> E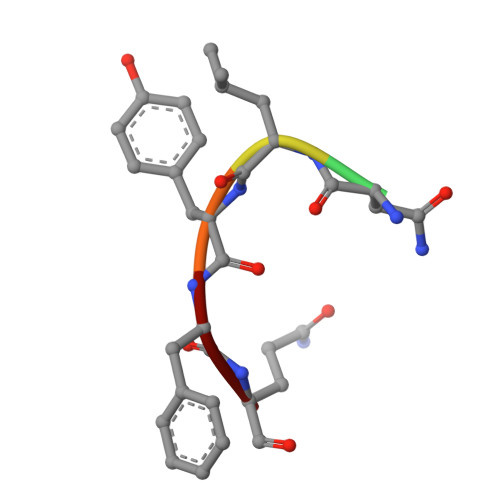NLYFQ> MKILVAVKQTAALEEDFEIREDGMDVD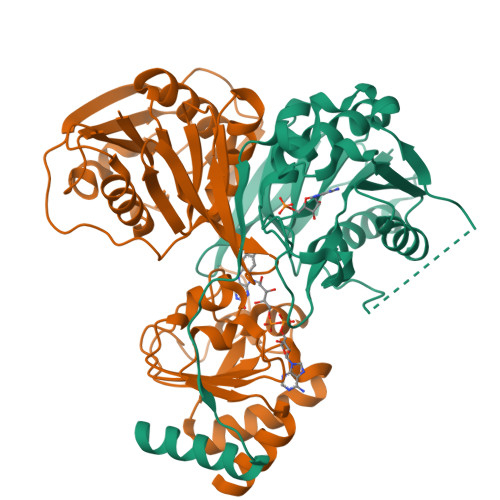EDFMMYDLNEWDDFSLEEAMKIKESSDTDVEVVVVSVGPDRVDESLRKCLAKGADRAVRVWDDAAEGSDAIVVGRILTEVIKKEAPDMVFAGVQSSDQAYASTGISVASYLNWPHAAVVADLQYKPGDNKAVIRRELEGGMLQEVEINCPAVLTIQLGINKPRYASLRGIKQAATKPIEEVSLADIGLSANDVGAAQSMSRVRRMYIPEKGRATMIEGTISEQAAKIIQIINEFKGA;> MSKILVIAEHRRNDLRPVSLELIGAANGLKKSGEDKVVVAVIGSQADAFVPALSVNGVDELVVVKGSSIDFDPDVFEASVSALIAAHNPSVVLLPHSVDSLGYASSLASKTGYGFATDVYIVEYQGDELVATRGGYNQKVNVEVDFPGKSTVVLTIRPSVFKPLEGAGSPVVSNVDAPSVQSRSQNKDYVEVGGGNDIDITTVDFIMSIGRGIGEETNVEQFRELADEAGATLCCSCPIADAGWLPKSRQVGQSGKVVGSCKLYVAMGISGSIQHMAGMKHVPTIIAVNTDPGASIFTIAKYGIVADIFDIEEELKAQLAA> VLGKPQTDPTLEWFLSHCHIHKYPSKSTLIHQGEKAETLYYIVKGSVAVLIKDEEGKEMILSYLN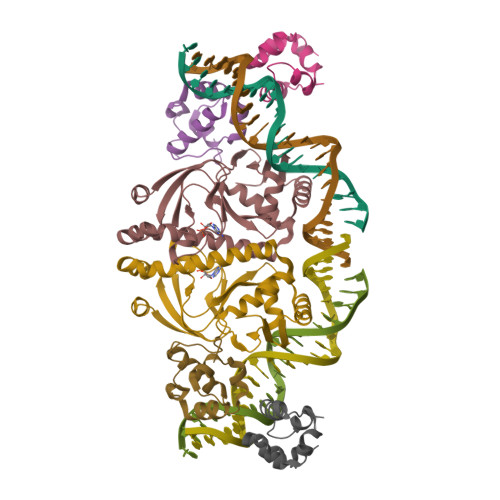QGDFIGELGLFEEGQERSAWVRAKTACEVAEISYKKFRQLIQVNPDILMRLSAQMARRLQVTSEKVGNLAFLDVTGRIAQTLLNLAKQPDAMTHPDGMQIKITRQEIGQIVGCSRETVGRILKMLEDQNLISAHGKTIVVYGTR;>KPEFDPILLRPVDDLELTVRSANCLKAEAIHYIGDLVQRTEVELLKTPNLGKKSLTEIKDVLASRGLSLGMRLENWPPASIADE[2x]> GPLGSDSDEMPSECISRRELEKGRISREEMETLS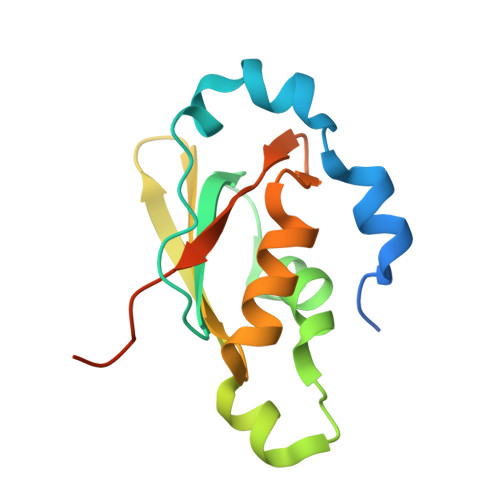VFRSYEPGEPNCRIYVKNLAKHVQEKDLKYIFGRYVDFSSETQRIMFDIRLMKEGRMKGQAFIGLPNEKAAAKALKEANGYVLFGKPMVVQFARSARPKQDPKEGKRKC(2~{R})-3-[3,4-bis(oxidanyl)phenyl]-2-oxidanyl-propanoic 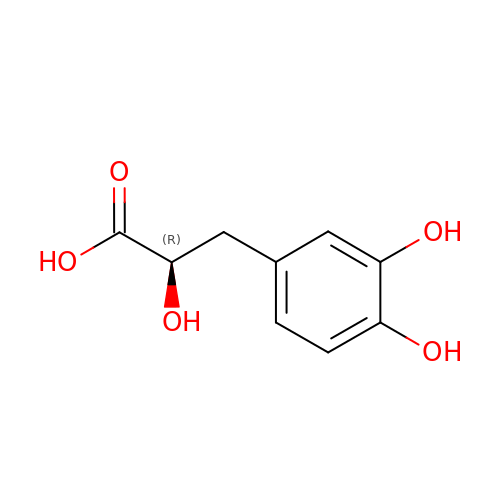acid | C9 H10 O5 | PAFLSMZLRSPALU-MRVPVSSYSA-N> HPYYLRSFLVVLKTVLENEDDMLLFDEQEKGIVTKFYQLSATGQKLYVRLFQRKLSWIKMTKLEYEEIALDLTPVIEELTNAGFLQTESELQELSEVLELLSAPELKSLAKTFHLVNPNGQKQQLVDAFLKLAKQRSVCTWGKNKPGIGAVILKRAKALAGQSVRICKGPRAVFSRILLLFSLTDSMEDEDAACGGQGQLSTVLLVNLGRMEFPSYTINRKTHIFQDRDDLIRYAAATHMLSDISSAMANGNWEEAKELAQCAKRDWNRLKNHPSLRCHEDLPLFLRCFTVGWIYTRILSRFVEILQRLHMYEEAVRELESLLSQRIYCPDSRGRWWDRLALNLHQHLKRLEPTIKCITEGLADPEVRTGHRLSLYQRAVRLRESPSCKKFKHLFQQLPEMAVQDVKHVTITGRLCPQRGMCKSVFVMEAGEAADPTTVLCSVEELALAHYRRSGFDQGIHGEGSTFSTLYGLLLWDIIFMDGIPDVFRNACQAFPLDLCTDSFFTSRRPALEARLQLIHDAPEESLRAWVAATWHEQEGRVASLVSWDRFTSLQQAQDLVSCLGGPVLSGVCRHLAADFRHCRGGLPDLVVWNSQSRHFKLVEVKGPNDRLSHKQMIWLAELQKLGAEVEVCHVV;>MFEARLVQGSILKKVLEALKDLINEACWDISSSGVNLQSMDSSHVSLVQLTLRSEGFDTYRCDRNLAMGV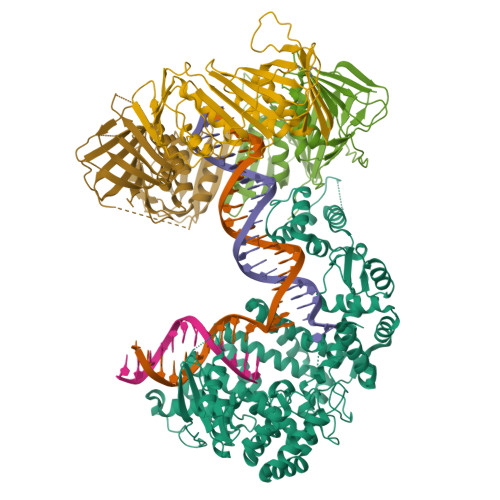NLTSMSKILKCAGNEDIITLRAEDNADTLALVFEAPNQEKVSDYEMKLMDLDVEQLGIPEQEYSCVVKMPSGEFARICRDLSHIGDAVVISCAKDGVKFSASGELGNGNIKLSQTSNVDKEEEAVTIEMNEPVQLTFALRYLNFFTKATPLSSTVTLSMSADVPLVVEYKIADMGHLKYYLAPKIE[3x]>MGSSHHHHHHSSGMSGCSKDSDSGFYEPEPIEEDPTPENPLPPGELDFEPEETRSFMVNPDATEETVALFYNLKLLSQNSFIVGQQDAFSSFYQDNAGDSDIKKMTGSDPGLLGSDFMFITDDLNDGTPSNWFFQQENQIRDDVLRAFDMGLVNVFCWHFREPFEGEHFYTSEMTQFQRENALKSILPGGENHDYYKQKLEKIASFTKSLVGSNGALVPIIFRPFHEFDGDWFWWGQSFCTIEEYIQLWQFTVTYLKNTLSVNNMLFAFSPDNRFFSESEYLARYPGDDFVDIMGMDNY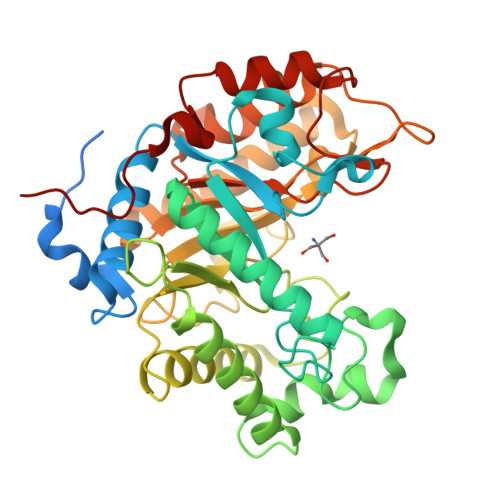GDFNNQGQAGVERANQKLKIVSDLAEERVKIASLTETGYFVTLSENGAIPGFFTNNLFEALTHNDVKIGFTMFWYNYQDTYCTPVPGLPSANDFMEFVSKPEVILADDLPEMYRLPPNS[2x]>[2x]ICSGPQNLAQELKAIGDQLQELQKKLIQGPNISQPRPLLTIETPRHLGEQLNARRKELGIDLYTLELQTGISTSTLKRLFKDPEQVKFGSVFAVANVLGVKLCIGE;>HRRVKVLLYGQVVGELSQNDSGFLFQYAHDYHGPAISISLPVAQRQFPSETLHPYFASLAPEGWLRQRYSQIQHRDENDLLGMLIDNGKNLLGAIQILPWEE[2x];>ANCRILLTPLNERDEQRGYSTQGLKRLSGTAKLNPRLGFTRTQFVQELPRQQKGMSISGYQPKLQLVLDEGEFRVVDHQGNFILKPSPADFPGLAENEHATMTLMSRLGFDVPVHGLLSFAPQSEEELEYAFVIRRYDRDNKGLPVHQEQLDGAMQITDKYGKTGNDNEQYVSYETLARFLVAHVNDNIAFKIDLFRRIVYAWLLGNNDMHLRNFGLVYSDGLTPALAPVYQFVSVAPYPEYFYSNYLALPLLTREEGGRE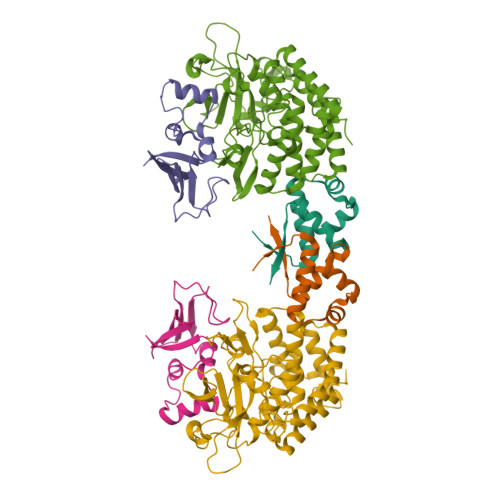LAPGFHSDYGEYIGQDFLLLGESMGLAPRLLEKLFQDIRKENAIVMETYEQSFMTQDHIQAVLQCYRHRLGLLHHHHHH[2x]> DKLDYFELFKEYLKKRE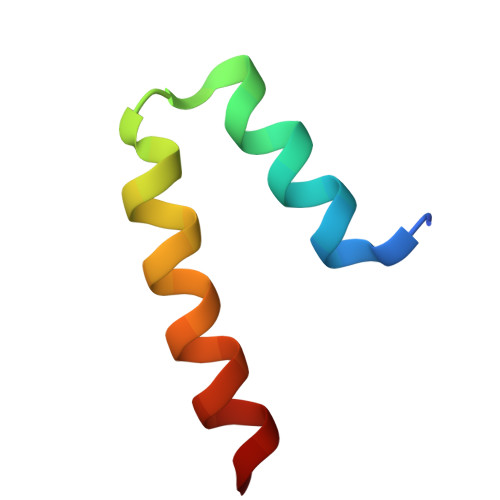ENHEKLLKILDELLDEVKKS>[4x]DEPGVATGNGQPVTGNWLAGASQGDGVPIPSQIADQLRGKEFKSWRDFREQFWMAVSKDPSALENLSPSNRYFVSQGLAPYAVPEEHLGSKEKFEIHHVVPLESGGALYNIDNLVIVTPKRHSEIHKELKLKRKEK;>[4x]MDIKNNLSDYTESEFLEIIEEFFKNKSGLKGSELEKRMDKLVKHFEEVTSHPRKSGVIFHPKPGFETPEGIVKEVKEWRAANGLPGFKAGLEHHHHHH

Immunity proteins protect the colicin producing, or “colicinogenic”, bacteria by binding and inactivating colicin nucleases with very high affinity (Kd ≈ 10− 14 M) and specificity; the discrimination in binding affinity between cognate and non-cognate nucleases by Im proteins can be up to 10 orders of magnitude. In the context of DNase bacteriocins, the HNH motif, which coordinates a single divalent metal ion within its centre, binds to the minor groove of genomic DNA causing random cleavages that overwhelm the DNA repair machinery of the cell and result in death within minutes of intoxication. The immunity protein associated with DNase colicins has an unusual mode of action; rather than binding directly to the DNase catalytic core, these proteins associate with the nuclease domain at an exosite adjacent to the enzyme active site. In this work, we have solved the first structures of the DNase domains of pyocins S2 and AP41 in complex with their cognate Im proteins, in addition to the structure of the isolated pyocin AP41 DNase domain.

Pyocin DNase–Im complexes were crystallised and structures solved to 2.0 Å and 1.8 Å for the pyocin AP41 DNase–ImAP41 and pyocin S2 DNase–ImS2 complexes, respectively. However, surprisingly, the relative domain positions in the AP41 DNase–Im complex superimpose well with the colicin E9 DNase–Im9 complex and do not exhibit the twisted relative domain positioning that is observed in the ColE7–Im7 complex. Compared with the colicin immunity proteins, ImAP41 loop 1 contains three additional amino acids and this is reflected in the more elaborate conformation it adopts (right). The first aromatic residue, Phe59, forms a parallel π-stacking interaction with Tyr722 within pyocin AP41 DNase domain in a manner similar to the Tyr in Im2 and ImS2. The PyoAP41–ImAP41 complex is stabilised by an orthogonal (T-shaped) π-stacking interaction between ImAP41 Phe59 and PyoAP41 Phe714. The second aromatic residue, His60, forms a hydrogen bond to the backbone carbonyl of Tyr722 making contacts equivalent to those of Im2 Tyr55 in the ColE2–Im2 complex and ImS2 Tyr56 in the PyoS2–ImS2 complex. In the alternate hotspot, represented by PyoAP41–ImAP41, the invariant Asp is replaced by a Gly that has very different physicochemical properties. A complementary substitution in the DNase, PyoAP41 Pro725, accommodates the vacated space in ImAP41 (right). However, the second water that is coordinated by the Asp side chain in Im2 and ImS2 is absent in the AP41 complex; the absence of the acidic side chain from ImAP41 removes this water-mediated interaction. The cognate AP41 complex is strengthened by two water-mediated intermolecular hydrogen bonds between the guanidinium group of ImAP41 Arg53 and the carboxylic acid of Glu726, the side chain of which occupies the position of the water in Im2 and ImS2.> AARYDDVLYFPASRYPETGAHISDAIKAGHADVCTIERSGADKRRQESLKGIPTKPGFDRDEWPMAMCEEGGKGASVRYVSSSDNRGAGSWVGNRLNGYADGTRILFIVQ

Here, we have characterized NucB, a biofilm-dispersing nuclease from a marine strain of Bacillus licheniformis, and present its crystal structure together with the biochemistry and a mutational analysis required to confirm its active site. When the secondary structure of the single stranded substrates were calculated, position 20 tended to occur at the boundary between predicted single and double stranded regions of the DNA. It has already been shown that BlNucB had no detectable activity against total RNA purified from the periodontitis-associated oral bacterium Veillonella parvula in comparison to the positive control, RNase A. Therefore, BlNucB is a Mn2+/Mg2+-dependent, non-specific endonuclease that can cleave both single- and double-stranded substrates, but with a preference for double stranded DNA. NucB, on the other hand, is necessary for the degradation of eDNA for the dispersal of bacterial biofilms. BlNucB diverges from this general description because glutamate replaces the histidine, and this glutamate is essential for biological activity; therefore BlNucB is the founding member of a novel subfamily of the His-Me finger nuclease superfamily.

To understand the molecular basis of its nuclease activity, the structure of BlNucB was solved by single wavelength anomalous dispersion (SAD) from the intrinsic sulphur atoms in the protein and refined to a resolution of 1.35 Å. Overall, BlNucB is a single, compact domain comprising five β-strands and three α-helices that forms a rough triangular pyramid with an approximate diameter of 25 Å. The core of the protein is formed by the five β-strands in a bipartite β-sheet, with β-strands with topological order 1, 5 and 2 separated from β-strands 3 and 4 by the β3-β4 loop that breaks the continuity of the β-sheet. The β3-β4 loop is stabilized in part by the formation of a disulphide bond between β2 residue Cys66 and the β3-β4 loop residue Cys100. Instead, the flat base of the pyramid contains a 15 Å deep, 10 Å wide, 20 Å long concave depression that is formed mostly by conserved amino acids. The base of the depression is predominantly negatively-charged, whereas the lips of the cavity are mostly positively-charged. The surface depression is of sufficient size to accommodate a single strand of DNA, presenting the scissile phosphodiester bond to the catalytic apparatus, whilst the lips of the cavity can interact with the DNA phosphate backbone. There is no metal ion bound in the apo structure of BlNucB reported here and, despite repeated attempts, we were unable to obtain diffracting crystals containing either bound divalent cations or oligodeoxynucleotides. As with other members of the His-Me finger family, BlNucB retains the metal-binding pocket, including the metal-chelator Asn117 and, as in Vvnendo, BlNucB encodes an acid (Asp93) immediately before Glu94 and located so that with minimal changes to the sidechain chi angles it can be positioned to co-ordinate directly to a bound divalent cation.> GAMAQQPVVRVGEWLVTPSINQISRNGRQLTLEPRLIDLLVFFAQHSGEVLSRDELIDNVWKRSIVTNHVVTQSISELRKSLKDNDED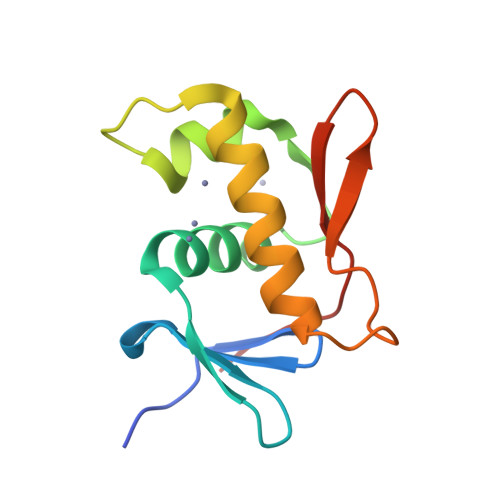SPVYIATVPKRGYKLMVPVIWY> GSKNIVNTSILSIVYKKDDLIDLSRYGAKINIGDRVYYDSIDKN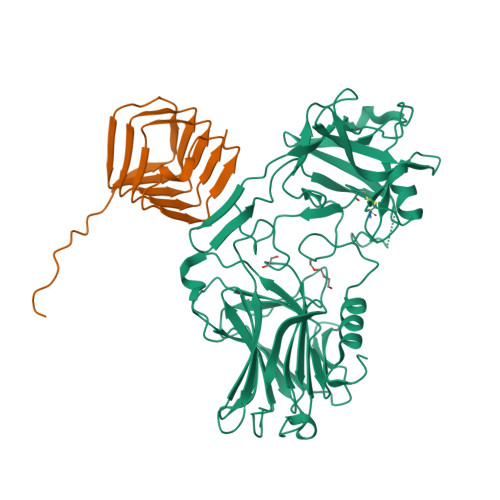QIKLINLESSTIEVILKNAIVYNSMYENFSTSFWIKIPKYFSKINLNNEYTIINCIENNSGWKVSLNYGEIIWTLQDNKQNIQRVVFKYSQMVNISDYINRWIFVTITNNRLTKSKIYINGRLIDQKPISNLGNIHASNKIMFKLDGCRDPRRYIMIKYFNLFDKELNEKEIKDLYDSQSNSGILKDFWGNYLQYDKPYYMLNLFDPNKYVDVNNIGIRGYMYLKGPRGSVVTTNIYLNSTLYEGTKFIIKKYASGNEDNIVRNNDRVYINVVVKNKEYRLATNASQAGVEKILSALEIPDVGNLSQVVVMKSKDDQGIRNKCKMNLQDNNGNDIGFIGFHLYDNIAKLVASNWYNRQVGKASRTFGCSWEFIPVDDGWGESSL;> MKKHHHHHHGSLVPRGSDVIKPLQSDEYALLTRNVERDKYANFTINFTMENQIHTGMEYDNGRFIGVKFKSVTFKDSVFKSCTFEDVTSVNTYFKNCTFIDTVFDNTDFEPYKFIDSEFKNCSFFHNKTGCQITFD> MSAKKIVLKSSDGESFEVEEAVALESQTIAHMVEDDCVDNGVPLPNVTSKILAKVIEYCKRHVEAAASKAEAVEGAATSDDDLKAWDADFMKIDQATLFELILAANYLNIKNLLDLTCQTVADMIKGKTPEEIRTTFNIKNDFTPEEEEEVRRENQWAFE;> MQKRIALSFPEEVLEHVFSFIQLDKDRNSVSLVCKSWYEIERWCRRKVFIGNCYAVSPATVIRRFPKVRSVELKGKPHFADFNLVPDGWGGYVYPWIEAMSSSYTWLEEIRLKRMVVTDDCLELIAKSFKNFKVLVLSSCEGFSTDGLAAIAATCRNLKELDLRESDVDDVSGHWLSHFPDTYTSLVSLNISCLASEVSFSALERLVTRCPNLKSLKLNRAVPLEKLATLLQRAPQLEELGTGGYTAEVRPDVYSGLSVALSGCKELRCLSGFWDAVPAYLPAVYSVCSRLTTLNLSYATVQSYDLVKLLCQCPKLQRLWVLDYIEDAGLEVLASTCKDLRELRVFPSEPFVMEPNVALTEQGLVSVSMGCPKLESVLYFCRQMTNAALITIARNRPNMTRFRLCIIEPKAPDYLTLEPLDIGFGAIVEHCKDLRRLSLSGLLTDKVFEYIGTYAKKMEM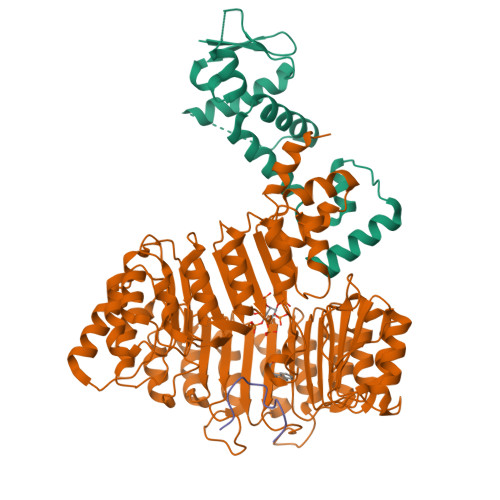LSVAFAGDSDLGMHHVLSGCDSLRKLEIRDCPFGDKALLANASKLETMRSLWMSSCSVSFGACKLLGQKMPKLNVEVIDERGAPDSRPESCPVERVFIYRTVAGPRFDMPGFVWNMDQDSTMRFSRQIITTNGL;> QVVGWPPVRNYRK> SYYHHHHHHLESTSLYKKAGLRMLIFTYKLERYIKNKILPKILVVPDRDKYQIKGSFRRRIPYITDIDIVNNVHPEYDDTNIYQRIVDLINSFTNDNQIKLIYVICGTDDRFLLTEYSDEEIEKIKILLNPTELVELNNVLSKYQDDLNKKVFYINEIIWDLYKLRWTSSEVLAGKKILRGGIEVSFQDVVKNNSILLLQYFVKIEYYPIGFDIAVRYKPINLITAYQNAAFYQLKLANYSKEYYFML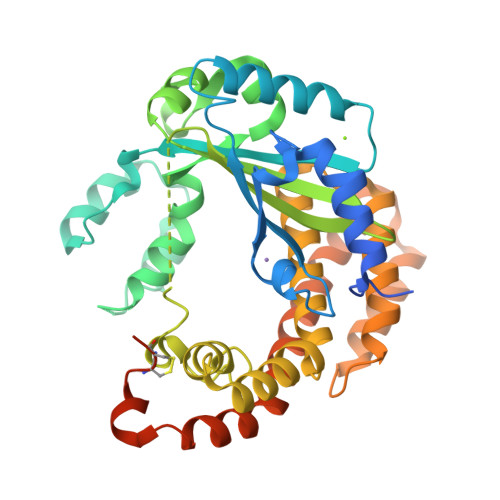FPLRFYFKNDPTISKQLEYIIETKFGLYKQLLVRIDSYRTIYESGNLDLDTAKSIIISIIKDIRKLNGIDMNIIDKIQEVSNNSAGQDKIIAWNTLLTQLYTNINKSVNKQSKKYFTRYINIIPKEDRKLCCLEEEHVLQSGGINFESTNFLTKKKLIY>[2x]MKYSQCLKGEVVMIPALAKKILHVTVGTLLVSSAASMMVYLNSMCHMAANSKTQQIQGDDNKDDKFPLAAISKVVTTLWAVDRLGPDYRFKTKLHVTPTANGSYDIHIEGSRDPLFGRNMSYFLISELNRMKITKIEKLTFDENFLLAWLAEEKPMIGGTTPKYDTVEQQASIVRATLTSSFATAISPGYY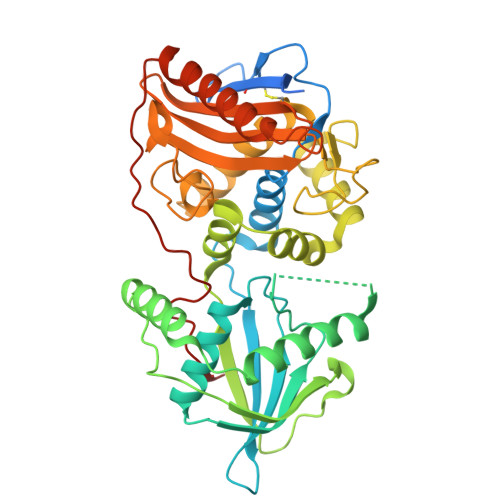TILKTKAARIGVQMSNRPKIDVRTISFVKKAEFQKNEKSTTMVLMSAPLKTILKRMNNQSNNYIADNLYWNLGGTEAFNAYIAGKMQADTSDIEFHNGSGNNEGSVAKPVYNEATCEMMIKVLYSLDKSLSAKGYDLSDVMAVAAKDKASTVGSYGGVMAGSTTAKTGSVNKAKTLMGSVSTKNGEIYFAVLMHTDYDKSRSDWGVASQQIKNKVSQLINQNGGPKAIKYTEQLPLPFDKYSYLTKANTITTEKK>SLRSDLINALYDENQKYDVCGIISAEGKIYPLGSDTKVLSTIFELFSRPIINKIAEKHGYIVEEPKQLNHYPDFTLYKPSEPNKKIAIDIKTTYTNKENEKIKFTLGGYTSFIRNNTKNIVYPFDQYIA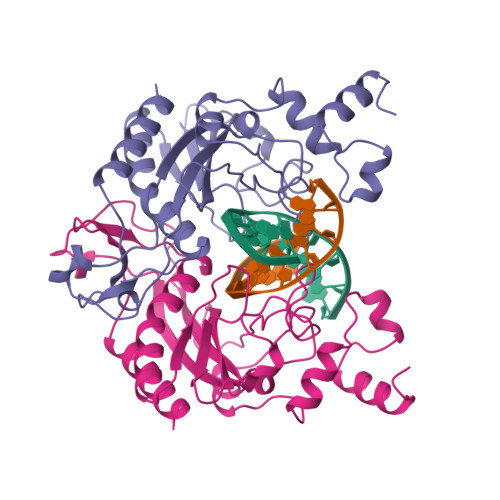HWIIGYVYTRVATRKSSLKTYNINELNEIPKPYKGVKVFLQDKWVIAGDLAGSGNTTNIGSIHAHYKDFVEGKGIFDSEDEFLDYWRNYERTSQLRNDKYNNISEYRNWIYRGRK[2x]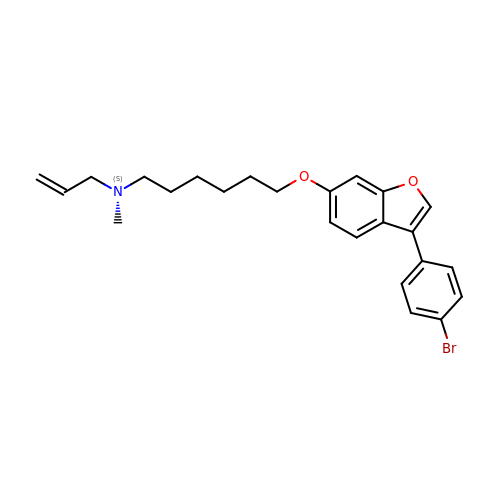ALLYL-{6-[3-(4-BROMO-PHENYL)-BENZOFURAN-6-YLOXY]-HEXYL-}-METHYL-AMIN | C24 H28 Br N O2 | JYNZIOFUHBJABQ-UHFFFAOYSA-N(2S)-2-AMINO-5-(3-METHYLPHENYL)-5,5-DIPHENYLPROPANOIC 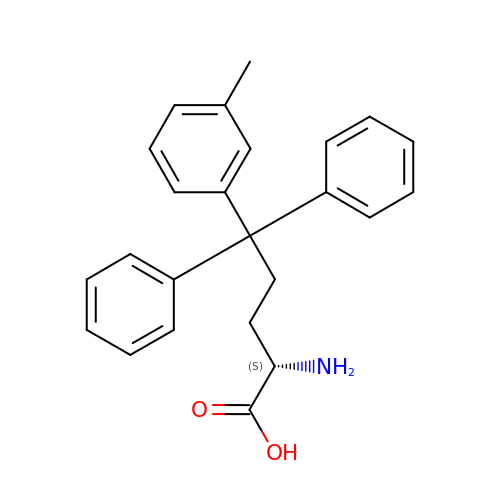ACID | C24 H25 N O2 | JXIGVUPYYZGRRZ-QFIPXVFZSA-N N-[(2S,3R)-3-hydroxy-1-(hydroxyamino)-1-oxobutan-2-yl]-4-(phenylethynyl)benzamide | C19 H18 N2 O4 | 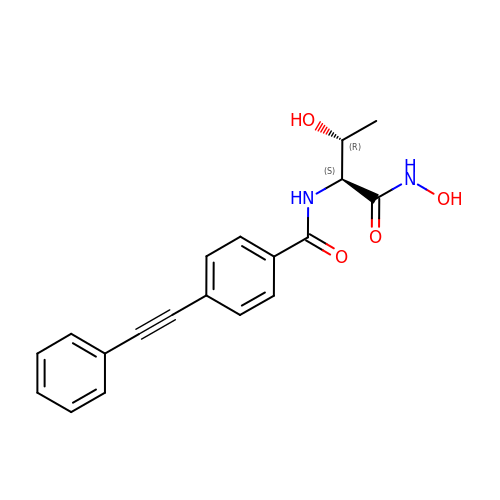SFYISUPIFOZKLQ-DYVFJYSZSA-N In this work, we exhaustively probe the ability of all 36 immobile HJ sequences to form DNA crystals in two different designed systems. Three separate self-assembling DNA crystal systems are described in this report: the “4 × 5” and “4 × 6” designs (collectively referred to as the 4 × N systems), and a third construct with a “scrambled” sequence variant of the 4 × 6 lattices. Self-assembly was mediated by three constituent oligonucleotides: (S1) containing four sequence repeats of either 5 or 6 bases; (S2) composed of 21 bases containing complementary regions to both (S1); and (S3) which forms the second junction crossover. The HJ serves as the fundamental component at the core of each unit, and the ultimate assembly of the full lattice is facilitated by the complementary 2-base sticky ends that tail each duplex.

The 4 × 5 system robustly crystallized with 75% of the junctions, and we obtained crystals in all but 9 of 36 sequences. Of the resulting structures, 18 exhibited P32 symmetry with average cell dimensions a = b = 68.85 Å c = 60.09 Å, with only nine retaining the original P3221 symmetry with average cell edges a = b = 68.17 Å c = 60.60 Å. Although the cell parameters between the two symmetries were virtually indistinguishable, the differences between the periodicity of the lattices is dramatic, with vastly different cavity sizes. While the highest resolution achieved for the J1 system was 3.1 Å, in roughly half of the crystals measured the resolutions were 3.05 Å or better, and as high as 2.9 Å (J6) and 2.75 Å (J19), for the P32 and P3221 symmetries, respectively. The P32 channels were treated as a hexagonal prism with 6.4 nm along each edge and a height measured from the top to the bottom of each block along with the average c-axis = 6.0 nm, with a resulting volume of ~639 nm3, a nearly 27-fold increase in cavity size relative to the P3221 lattices. However, in the majority of the crystal structures reported here, the cacodylate anion indeed fits best into the electron density map of our X-ray structures, due to the presence of sodium cacodylate in the crystallization solution.

> GAGCAGACAAG;> ACTTCACTCA;> CTAGT;> TCTGAGTGATGTCTGC>AQVINTFDGVADYLQTYHKLPDNYITKSEAQALGWVASKGNLADVAPGKSIGGDIFSNREGKLPGKSGRTWREAD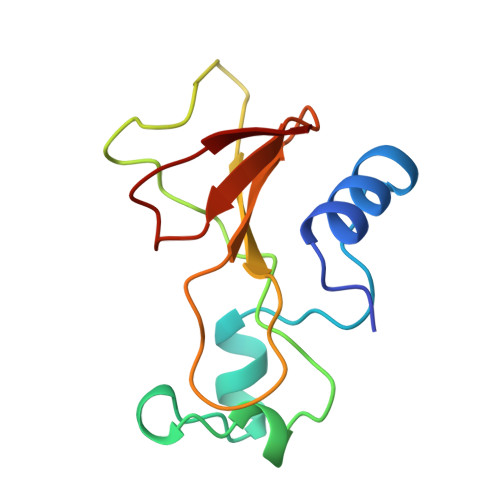INYTSGFRNSDRILYSSDWLAYKTTDHYQTFTKIR[3x]Here, we demonstrated that the BAH domain-containing protein anti-silencing 1 (ASI1)-IMMUNOPRECIPITATED PROTEIN 3 (AIPP3) and two PHD domain-containing proteins AIPP2/PARALOG OF AIPP2 (PAIPP2) could form a BAH–PHD module to read H3K27me3 and unmethylated H3K4, respectively, and coordinate in implementing transcriptional repression of hundreds of genes, particularly those development and stress-responsive genes in Arabidopsis, such as the florigen gene FT and the RNA silencing effector gene AGO5. We also revealed that the BAH–PHD module represses the release of Pol II from TSS regions by cooperating with CPL2, a known plant-specific Pol II carboxyl terminal domain (CTD)-Ser5 phosphatase. Moreover, consistent with the histone pull-down result, AIPP3-BAH has a preference for the higher methylation level in H3K27. Thus, the evidence above fully demonstrated that AIPP3-BAH is a H3K27me3-reader module. In this model, the BAH–PHD bivalent histone reader recognizes H3K27me3, and unmodified H3K4 marks and recruits CPL2 to dephosphorylate the Ser5P of Pol II CTD, resulting in the inhibition of Pol II release from a transcriptional initiation state to elongation.

To gain molecular insight into the interaction between the AIPP3-BAH domain and H3K27me3, we successfully determined the crystal structure of the AIPP3-BAH domain in complex with an H3K27me3 peptide at a resolution of 2.4 Å. Overall, the AIPP3-BAH domain has a classic β-barrel structure that is similar to other reported BAH domain structures. The H3K27me3 peptide has a good electron density map and a β-strand-like extended conformation. The peptide is captured by a negatively charged cavity that is formed on the surface of the AIPP3-BAH domain with extensive hydrophobic and hydrophilic interactions. In detail, the three aromatic residues of the AIPP3-BAH domain, Tyr149, Trp170, and Tyr172, form an aromatic cage to accommodate the trimethyl-lysine of the H3K27me3 peptide, and it resembles other typical methyl-lysine-reading histone readers. At the N-terminus, the H3A25 forms two main chain–main chain hydrogen bonds with the AIPP3 Val140 and Glu142. In the middle, the AIPP3 residues Trp170, Tyr172, His198, and Asp200 form an extensive hydrogen-binding network with H3S28, which further fixes the imidazole ring of His198 in a special rotamer state that is parallel with the prolyl ring of H3P30. This parallel alignment of the two rings enables the CH-π, and stacking interactions between AIPP3 His198 and H3P30, which resemble the recognition of H3K27me3 by the EBS and SHL BAH domains with conserved key residues. In the C-terminus, H3G33 interacts with AIPP3 Val240 through a main chain–main chain hydrogen bond.

> SGKGKGKRTHFNQFAYDGNTYDLEVPVLLVPEDKSQKPYVAIIKDITQTKDGSMMILGQWFYRPEEAEKRGGGNWQSSDTRELFYSFHRDEVPAESVMHRCVVYFVPAHKQLPKRKNNPGFIVRKVYDTVEKKLWKLTDKDYEDSKQREIDVLVKKTMNVLGDLPDLES;> LATKAARKSAPATGGVKK> GEKTYVKRLVKILLLGAGESGKSTFLKQMRIIHGQDFDQRAREEFRPTIYSNVIKGMRVLVDAREKLHIPWGDNKNQLHGDKLMAFDTRAPMAAQGMVETRVFLQYLPAIRALWEDSGIQNAYDRRREFQLGESVKYFLDNLDKLGVPDYIPSQQDILLARRPTKGIHEYDFEIKNVPFKMVDVGGQRSERKRWFECFDSVTSILFLVSSSEFDQVLMEDRQTNRLTESLNIFETIVNNRVFSNVSIILFLNKTDLLEEKVQVVSIKDYFLEFEGDPHCLRDVQKFLVECFRGKRRDQQQRPLYHHFTTAINTENIRLVFRDVKDTILHDNLKQL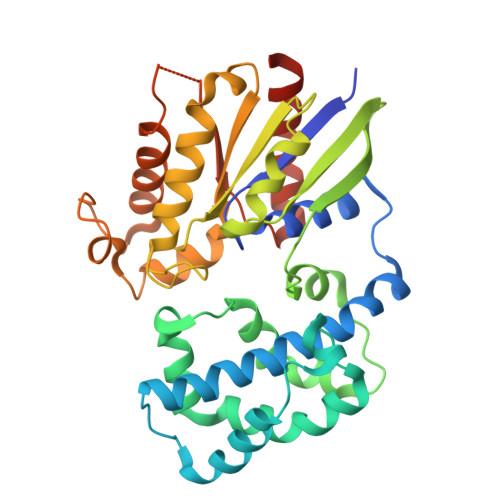MLQ[2-[tert-butyl-(phenylmethyl)amino]-2-oxidanylidene-ethyl] 4-bromanyl-5-nitro-furan-2-carboxylate 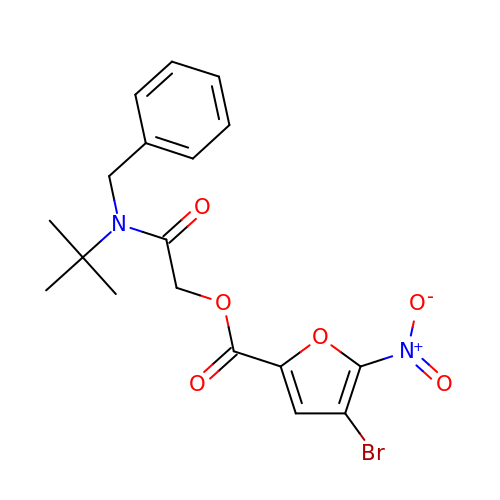| C18 H19 Br N2 O6 | ZLXQPKWHPMMLFG-UHFFFAOYSA-N>GTATAT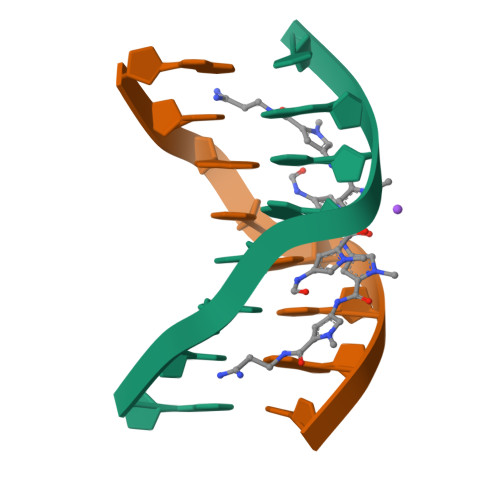AC[4x]> GMAAADGDDSLYPIAVLIDELRNEDVQLRLNSIKKLSTIALALGVERTRSELLPFLTDTIYDEDEVLLALAEQLGTFTTLVGGPE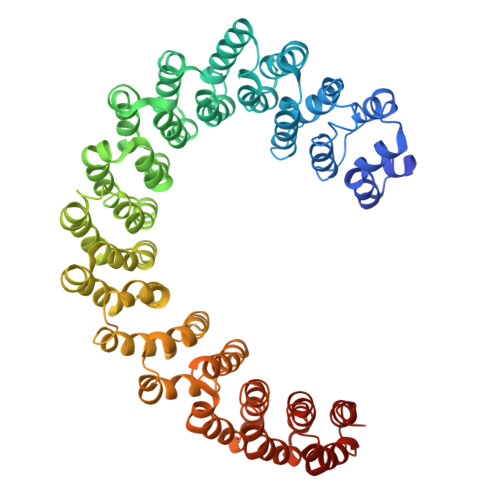YVHCLLPPLESLATVEETVVRDKAVESLRAISHEHSPSDLEAHFVPLVKRLAGGDWFTSRTSACGLFSVCYPRVSSAVKAELRQYFRNLCSDDTRMVRRAAASKLGEFAKVLELDNVKSEIIPMFSNLASDEQDSVRLLAVEACVNIAQLLPQEDLEALVMPTLRQAAEDKSWRVRYMVADKFTELQKAVGPEITKTDLVPAFQNLMKDCEAEVRAAASHKVKEFCENLSADCRENVIMTQILPCIKELVSDANQHVKSALASVIMGLSPILGKDNTIEHLLPLFLAQLKDECPEVRLNIISNLDCVNEVIGIRQLSQSLLPAIVELAEDAKWRVRLAIIEYMPLLAGQLGVEFFDEKLNSLCMAWLVDHVYAIREAATSNLKKLVEKFGKEWAHATIIPKVLAMSGDPNYLHRMTTLFCINVLSEVCGQDITTKHMLPTVLRMAGDPVANVRFNVAKSLQKIGPILDNSTLQSEVKPILEKLTQDQDVDVKYFAQEALTVLSLA> AKQFTKCELSQLLKDIDGYGGIALPELICTMFHTSGYDTQAIVENNESTEYGLFQISNKLWCKSSQVPQSRNICDISC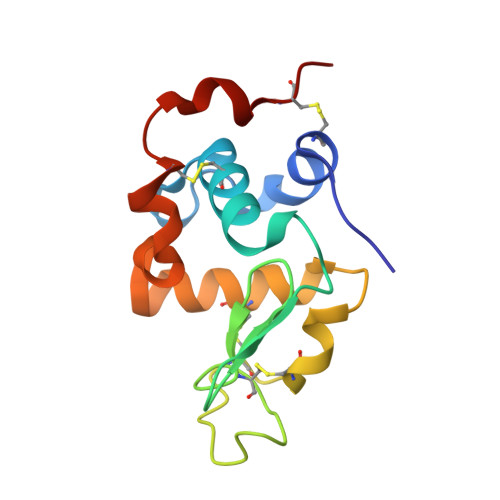DKFLDDDITDDIMCAKKILDIKGIDYWLAHKALCTEKLEQWLCEKL>[4x]SRPLSDQEKRKQISVRGLAGVENVTELKKNFNRHLHFTLVKDRNVATPRDYYFALAHTVRDHLVGRWIRTQQHYYEKDPKRIYYLSLEFYMGRTLQNTMVNLALE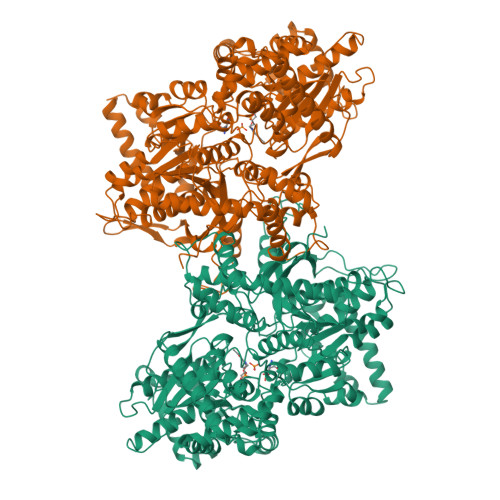NACDEATYQLGLDMEELEEIEEDAGLGNGGLGRLAACFLDSMATLGLAAYGYGIRYEFGIFNQKICGGWQMEEADDWLRYGNPWEKARPEFTLPVHFYGRVEHTSQGAKWVDTQVVLAMPYDTPVPGYRNNVVNTMRLWSAKAPNDFNLKDFNVGGYIQAVLDRNLAENISRVLYPNDNFFEGKELRLKQEYFVVAATLQDIIRRFKSSKFGCRDPVRTNFDAFPDKVAIQLNDTHPSLAIPELMRVLVDLERLDWDKAWEVTVKTCAYTNHTVIPEALERWPVHLLETLLPRHLQIIYEINQRFLNRVAAAFPGDVDRLRRMSLVEEGAVKRINMAHLCIAGSHAVNGVARIHSEILKKTIFKDFYELEPHKFQNKTNGITPRRWLVLCNPGLAEIIAERIGEEYISDLDQLRKLLSYVDDEAFIRDVAKVKQENKLKFAAYLEREYKVHINPNSLFDVQVKRIHEYKRQLLNCLHVITLYNRIKKEPNKFVVPRTVMIGGKPAPGYHMAKMIIKLITAIGDVVNHDPVVGDRLRVIFLENYRVSLAEKVIPAADLSEQISTAGTEASGTGNMKFMLNGALTIGTMDGANVEMAEEAGEENFFIFGMRVEDVDRLDQRGYNAQEYYDRIPELRQIIEQLSSGFFSPKQPDLFKDIVNMLMHHDRFKVFADYEEYVKCQERVSALYKNPREWTRMVIRNIATSGKFSSDRTIAQYAREIWGVEPSRQRLPAPDEKIP1-(3,4,5-trihydroxyphenyl)hexan-1-one | C12 H16 O4 | 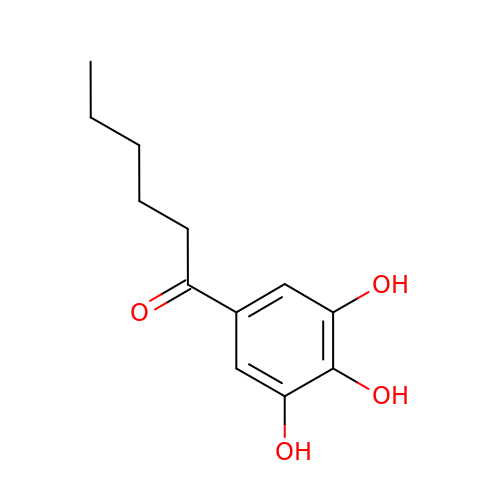IFYDUMLMLPWDRV-UHFFFAOYSA-N>[2x]SNASEPVTIVLSQMGWVRSAKGHDIDAPGLNYKAGDSFKAAVKGKSNQPVVFVDSTGRSYAIDPITLPSARGQGEPLTGKLTLPPGATVDHMLMESDDQKLLMASDAGYGFVCTF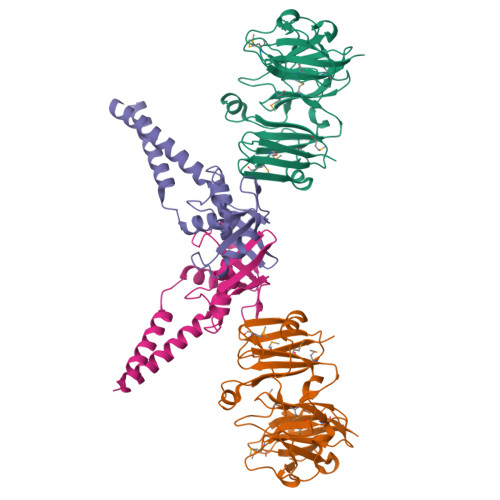NDLVARNRAGKALITLPENAHVMPPVVIEDASDMLLAITQAGRMLMFPVSDLPQLSKGKGNKIINIPSAEAARGEDGLAQLYVLPPQSTLTIHVGKRKIKLRPEELQKVTGERGRRGTLMRGLQRIDRVEIDSPRRASSGDSEE;>[2x]SNAERDEVGARKNAVDEEIERLSQPGGSEDQRLNALAERFGGVLLSEIYDDVSLEDAPYFSALYGPSRHAIVVPDLSQVTEHLEGLTDCPEDLYLIEGDPQSFDDSVFSVDELEKAVVVKIADRQWRYSRFPEVPLFGRAARESRIESLHAEREVLSERFATL>[8x]MAHHHHHHGAQQDAFVPLVRSMADRLNTADQ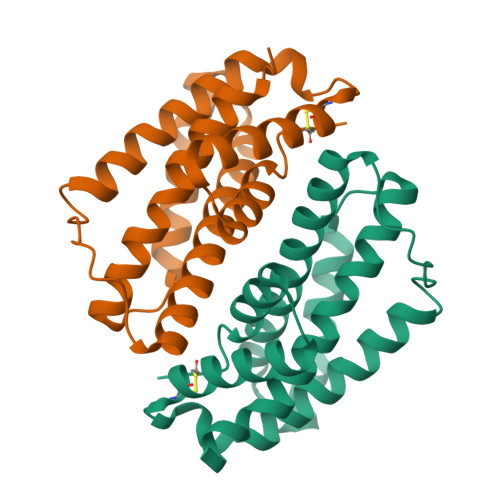VALSKWDTGQPVYDGQREAQVIANAATMASEYGLTAEDAINIFSDQVEANKEVQYALLNNWRRQGDAPATPRQSLAGVIRPILDKLQASIMQNLQSVAPLRSIADCHALVASAVGQVAEQASLDVLHRAALDRAVARICVKS> APLAAMDECADEGGRPQRCMPEFVNAAFNVTVVATNTCGTPPEEYCVQTGVTGVTKSCHLCDAGQQHLQHGAAFLTDYNNQADTTWWQSQTMLAGVQYPNSINLTLHLGKAFDITYVRLKFHTSRPESFAIYKRTREDGPWIPYQYYSGSCENTYSKANRGFIRTGGDEQQALCTDEFSDISPLTGGNVAFSTLEGRPSAYNFDNSPVLQEWVTATDIRVTLNRLNTFGDEVFNEPKVLKSYYYAISDFAVGGRCKCNGHASECVKNEFDKLMCNCKHNTYGVDCEKCLPFFNDRPWRRATAESASECLPCDCNGRSQECYFDPELYRSTGHGGHCTNCRDNTDGAKCERCRENFFRLGNTEACSPAAAHHHHHH

The laminins constitute a family of heterotrimeric glycoproteins. The short arms consist of one chain each and are composed of a distal laminin N-terminal (LN) domain followed by long tandem repeats of laminin-type epidermal growth factor-like (LE) domains, interrupted by one or two globular domains of unknown function. The LN domains are crucial for laminin polymerisation into a cell-associated two-dimensional network. Here, we report crystal structures of the N-terminal regions of the laminin β1 and γ1 chains, which define the common and unique features of laminin short-arm tips and reveal likely interaction sites for laminin polymerisation.

The diffraction limit of the trigonal crystals was limited to ∼3.8 Å in the c* direction, but extended beyond 3.2 Å in the directions normal to c*. A significant difference between the laminin β1 and γ1 structures is the presence of a calcium ion in the γ1 LN domain. The calcium ion is bound at the C-terminus of a short α-helix and co-ordinated by the side chains of Asp106 and Thr114, as well as three main chain carbonyl oxygens assume that the co-ordination shell is completed by water molecules bridging to the side chains of Asn108 and/or Asp277. An equivalent calcium site is present in netrins G1 and G2, but in these proteins there is a direct bond to the metal ion from a glutamic acid replacing Asn108 of laminin β1. Equilibrium dialysis and dot blot experiments with proteolytic laminin-111 fragments suggested the presence of a calcium binding site in the γ1 chain, and little calcium binding to the α1 and β1 chains. This result is entirely consistent with our crystal structures, which show a calcium site only in the γ1 domain. Furthermore, the partial co-ordination shell of this calcium ion is consistent with the relatively high dissociation constant of 55 µM determined by equilibrium dialysis. The calcium-binding loop in the γ1 LN domain does not contribute to the conserved patch on the β6-β3-β8 sheet, but it is adjacent to it. Whether the calcium ion bound to the γ1 LN domain is responsible for the calcium-dependence of laminin polymerisation remains to be seen. The conserved patch in the γ1 and γ3 chains includes less of the top surface of the LN domain, but is otherwise very similar to that of the β chain subfamily.> GSHMLETEEEEEEGAGATLSRGPAFPGMGSEELRLASFYDWPLTAEVPPELLAAAGFFHTGHQDKVRCFFCYGGLQSWKRGD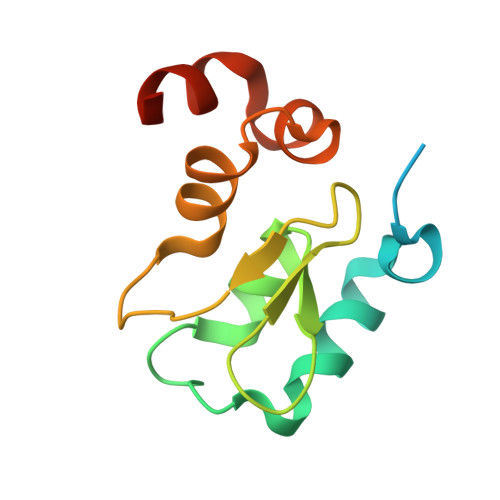DPWTEHAKWFPGCQFLLRSKGQEYINNIHLTHSL>MIRLYPEQLRAQLNEGLRAAYLLLGNDPLLLQESQDAVRQVAAAQGFEEHHTFSIDPNTDWNAIFSLCQAMSLFASRQTLLLLLPENGPNAAINEQLLTLTGLLHDDLLLIVRGNKLSKAQENAAWFTALANRSVQVTCQTPEQAQLPRWVAARAKQLNLELDDAANQVLCYCYEGNLLALAQALERLSLLWPDGKLTLPRVEQAVNDAAHFTPFHWVDALLMGKSKRALHILQQLRLEGSEPVILLRTLQRELLLLVNLKRQSAHTPLRALFDKHRVWQNRRGMMGEALNRLSQTQLRQAVQLLTRTELTLKQDYGQSVWAELEGLSLLLCHKPLADVFIDG[2x];>MSYQVLARKWRPQTFADVVGQEHVLTALANGLSLGRIHHAYLFSGTRGVGKTSIARLLAKGLNCETGITATPCGVCDNCREIEQGRFVDLIEIDAASRTKVEDTRDLLDNVQYAPARGRFKVYLIDEVHMLSRHSFNALLKTLEEPPEHVKFLLATTDPQKLPVTILSRCLQFHLKALDVEQIRHQLEHILNEEHIAHEPRALQLLARAAEGSLRDALSLTDQAIASGDGQVSTQAVSAMLGTLDDDQALSLVEAMVEANGERVMALINEA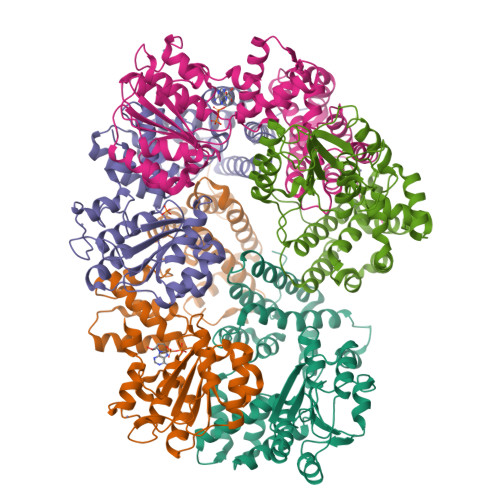AARGIEWEALLVEMLGLLHRIAMVQLSPAALGNDMAAIELRMRELARTIPPTDIQLYYQTLLIGRKELPYAPDRRMGVEMTLLRALAFHPRMPLPEP[6x];>[2x]MRWYPWLRPDFEKLVASYQAGRGHHALLIQALPGMGDDALIYALSRYLLCQQPQGHKSCGHCRGCQLMQAGTHPDYYTLAPEKGKNTLGVDAVREVTEKLNEHARLGGAKVVWVTDAALLTDAAANALLKTLEEPPAETWFFLATREPERLLATLRSRCRLHYLAPPPEQYAVTWLSREVTMSQDALLAALRLSAGSPGAALALFQGDNWQARETLCQALAYSVPSGDWYSLLAALNHEQAPARLHWLATLLMDALKRHHGAAQVTNVDVPGLVAELANHLSPSRLQAILGDVCHIREQLMSVTGINRELLITDLLLRIEHYLQPGVVLPVPHL>MGRASVGRMIGGIGRFYIQMCTELKLSDYDGRLIQNSITIERMVLSAFDERRNKYLEEHPSAGKDPKKTGGPIYRRVDGKWMRELILYDKEEIRRVWRQANNGEDATAGLTHIMIWHSNLNDATYQRTRALVRTGMDPRMCSLMQGSTLPRRSGAAGAAVKGVGTIAMELIRMIKRGINDRNFWRGENGRRTRVAYERMCNILKGKFQTAAQRAMMDQVRESRNPGNAEIEDLIFLARSALILRGSVAHKSCLPACVYGLAVASGHDFERE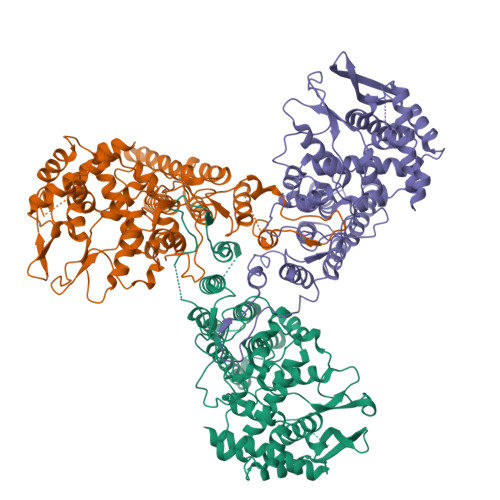GYSLVGIDPFKLLQNSQVVSLMRPNENPAHKSQLVWMACHSAAFEDLRVSSFIRGKKVIPRGKLSTRGVQIASNENVEIMDSNTLELRSRYWAIRTRSGGNTNQQKASAGQISVQPTFSVQRNLPFERATVMAAFSGNNEGRTSDMRTEVIRMMESAKPEDLSFQGRGVFELSDEKATNPIVPSFDMSNEGSYFF[3x]>QDSTSDLIPAPPLSKVPLQQNFQDNQFHGKWYVVGRAGNTGLREDKDPGKMFATIYELKEDKSYNVTYVWFGQKKCMYSIGTFVPGSQPGEFTLGNIKSAPGRTSWLVRVVSTNYNQHAMVFFKSVTQNREGFAITLYGRTKELTSELKENFIRFSKSLGLPENHIVFPVPIDQCIDGSAHHHHHH[2x];>[2x]ASWSHPQFEKGAELPAQKWWHTGALYRIGDLQAFQGHGAGNLAGLKGRLDYLSSLKVKGLVLGPIHKNQKDDVAQTDLLQIDPNFGSKEDFDSLLQSAKKKSIRVILDLTPNYRGENSWFSTQVDTVATKVKDALEFWLQAGVDGFQVRDIENLKDASSFLAEWQNITKGFSEDRLLIAGTNSSDLQQILSLLESNKDLLLTSSYLSDSGSTGEHTKSLVTQYLNATGNRWCSWSLSQARLLTSFLPAQLLRLYQLMLFTLPGTPVFSYGDEIGLDAAALPGQPMEAPVMLWDESSFPDIPGAVSANMTVKGQSEDPGSLLSLFRRLSDQRSKERSLLHGDFHAFSAGPGLFSYIRHWDQNERFLVVLNFGDVGLSAGLQASDLPASASLPAKADLLLSTQPGREEGSPLELERLKLEPHEGLLLRFPYAA

Structurally, CD98hc is a type-II-transmembrane glycoprotein which is disulfide-linked to one of six known multi-pass CD98 light chains (CD98lc), all of which are permease-type amino acid transporters with different specificities 3, namely Lat-1 4, Lat-2 5, y+Lat-1 6, y+Lat-2 7, asc-1 8 and xCT 9. First, it acts as a molecular chaperone for membrane trafficking, stabilization and proper function of the CD98lc 10, 11, thus boosting the transport of amino acids and contributing to cell survival and growth. Second, CD98hc directly contributes to intracellular integrin signaling and is involved in integrin-mediated cell to cell interactions via cellular adhesion molecules, such as VCAM-1, thereby influencing cell growth, survival, spreading and migration 15-19. Anticalins constitute an emerging class of artificial binding proteins obtained by combinatorial design based on the compact and robust human lipocalin scaffold 48.

To identify the epitope region and to understand the structural mechanisms of the tight molecular interaction between P3D11 and the CD98hc ectodomain, we crystallized this lipocalin variant in complex with hCD98hcED (carrying an N-terminal Strep-tag II) after isolation of the 1:1 complex via SEC. Crystals belonged to the space group C2, with two complexes per asymmetric unit, allowing collection of a synchrotron X-ray data set and refinement of the structure to a resolution of 1.8 Å. The engineered lipocalin binds to a membrane-distal part of hCD98hcED via the four variable loops #1-#4 at the open end of its β-barrel. The β-barrel axis of P3D11 is tilted by ~45° with regard to the TIM barrel axis of hCD98hcED. The contact interface between both proteins involves a buried surface area (BSA) of 1473 Å2 (1424 Å2 on the side of the lipocalin and 1521 Å2 on the one of hCD98hcED) as well as 15 hydrogen bonds and 3 salt bridges, resulting in the largest interface observed for Anticalin•protein complexes thus far 71. The interaction is favored by electrostatics as P3D11 is positively charged, which complements the predominantly negatively charged epitope on hCD98hcED, also reflecting the calculated pI values of 8.8 and 5.2 for P3D11 and hCD98hcED, respectively. The epitope of hCD98hcED essentially comprises two loops, L1 (residues 128-137) and L2 (374-404), which follow on the first and the eighth β-strand of the TIM barrel, respectively. Almost 75% of the contact interface is contributed by L2, which penetrates deeply into the binding pocket of the engineered lipocalin, while L1 contributes approximately 20% to the total BSA. Interestingly, binding of P3D11 causes an induced fit on the side of hCD98hcED.2-propylpyrimidin-4-amine | C7 H11 N3 | 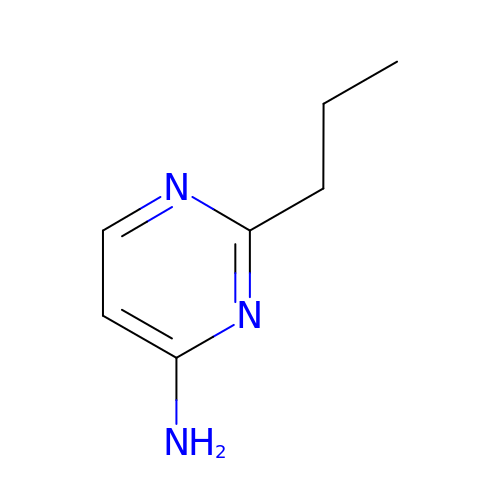BTMCCOMLYMKBFL-UHFFFAOYSA-N> MADVAGTSNRDFRGREQRLYNSEQYNYNNSLNGEVSLWVYAYYSDGSVLVRNCNSQYKVGISECFKSLKEVRVGQNNDPYDEQEVNNGVYYPNGGEPTKFHSNAKPRAIQIIFS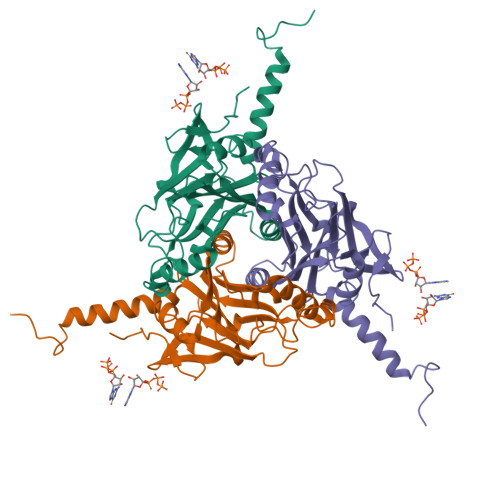PSVNVHTIKMAKGNSVSIPKDYLQRSHPWEATGVKYRKIHVDGEIVGYSHYFELPHEYNSISLSVSGVHKNPSSYNVAAPHNIMDVFQSCDLALKFSNRYWCELELINHYISAYAYPYLDINNHKYGVPLNGRQ> MVVSENVVSAPMPGKVLRVLVRVGDRVRVGQGLLVLEAMKMENEIPSPRDGVVKRILVKEGEAVDTGQPLIE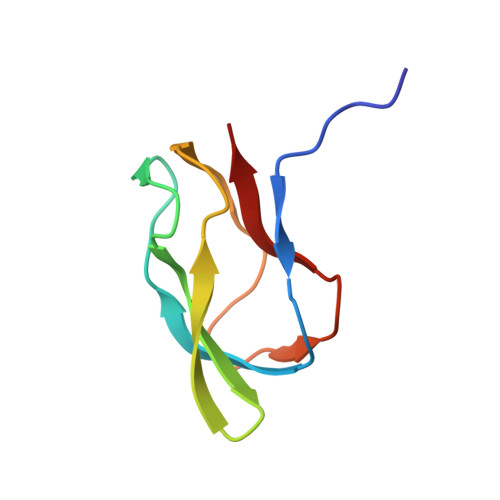LG Here we investigated the aminopeptidase, P. aeruginosa aminopeptidase (PaAP) from P. aeruginosa, which is highly abundant in the biofilm matrix. PaAP is associated with biofilm development and contributes to nutrient recycling. We confirmed that post-translational processing was required for activation and PaAP is a promiscuous aminopeptidase acting on unstructured regions of peptides and proteins. PaAP contains an M28 Zn peptidase domain (residues 44–116 and 274–510) and a PA domain (residues 117–273).

Guided by the structure of PaAP, we designed a cyclic peptide (cyclic-ERWGHDFIK) cyclized via an isopeptide bond between the glutamate and lysine side chains. Cyclic-ERWGHDFIK was a potent inhibitor of PaAP with a KI of 22.8 nM, which is ~440-fold lower than the linear peptide. Moreover, cyclic-ERWGHDFIK was not degraded when incubated overnight with PaAP. The structure of PaAP_T in complex with cyclic-ERWGHDFIK (PaAP_T(ERWGHDFIK)) was solved to confirm enzyme–inhibitor interactions. The structure of PaAP_T(ERWGHDFIK) is comparable to the structure of full-length PaAP, adopting the same closed/inactive conformation (RMSD = 0.3610 Å over 934 residues). Cyclic-ERWGHDFIK was predictably bound in the groove between the PA and peptidase domain, almost identical to the C-terminus bound in the full-length structure. Complete electron density was visible for the inhibitor, including the side chain linkage between K and E, which is shown in the omit map in Supplementary Fig. 6c. The inhibitor complex structure suggests inhibitor binding induces a conformational change, stabilizing the closed conformation and blocking access to the active site. Inhibition showed no time dependence, pointing toward this conformational change being a single-step process.

>[2x]SEAQQFTEFWTPGKPNPSICKSPLLVSTPLGLPRCLQASNVVKRLQKLEDIASLNDGNRAAATPGYQASVDYVKQTLQKAGYKVSVQPFPFTAYYPKGPGSLSATVPQPVTYEWEKDFTYLSQTEAGDVTAKVVPVDLSLGAGNTSTSGCEAEDFANFPAGSIALIQRGTCNFEQKAENAAAAGAAGVIIFNQGNTDDRKGLENVTVGESYEGGIPVIFATYDNGVAWSQTPDLQLHLVVDVVRKKTETYNVVAETRRGNPNNVVMVGAHLDSVFEGPGINDNGSGSAAQLEMAVLLAKALPVNKVRFAWWGAEEAGLVGSTHYVQNLAPEEKKKIKAYLNFDMIGSPNFGNFIYDGDGSDFGLQGPPGSAAIERLFEAYFRLRGQQSEGTEIDFRSDYAEFFNSGIAFGGLFTGAEGLKTEEQAQKYGGTAGKAYDECYHSKCDGIANINQDALEIHSDAMAFVTSWLSLSTKVVDDEIAAAGQKLVPR;>ERWGHDFIK[2x]> MFFYNTDFRMGSISAANAEFCFDVFNELKVQHT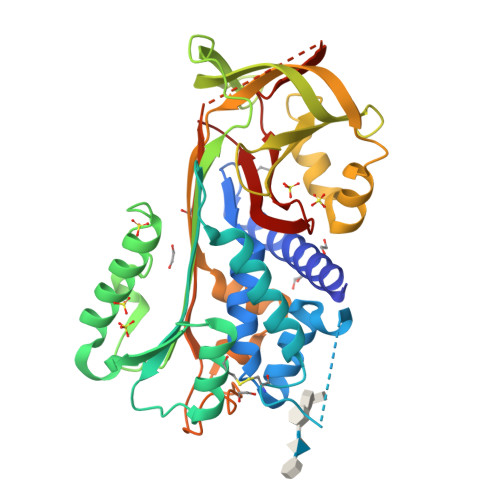NENILYSPLSIIVALAMVYMGARGNTEYQMEKALHFDSIAGLGGSTQTKVQKPKCGKSVNIHLLFKELLSDITASKANYSLRIANRLYAEKSRPILPIYLKCVKKLYRAGLETVNFKTASDQARQLINSWVEKQTEGQIKDLLVSSSTDLDTTLVLVNAIYFKGMWKTAFNAEDTREMPFHVTKEESKPVQMMCMNNSFNVATLPAEKMKILELPFASGDLSMLVLLPDEVSGLERIEKTINFEKLTEWTNPNTMEKRRVKVYLPQMKIEEKYNLTSVLMALGMTDLFIPSANLTGISSAESLKISQAVHGAFMELSEDGIEMAGSTGVIEDIKHSPELEQFRADHPFLFLIKHNPTNTIVYFGRYWSP> NIPFTDNLLFSGQVLYGDGRLTAKNHQLVMQGDCNLVLYGGKYGWQSNTHGNGEHCFLRLNHKGELIIKDDDFK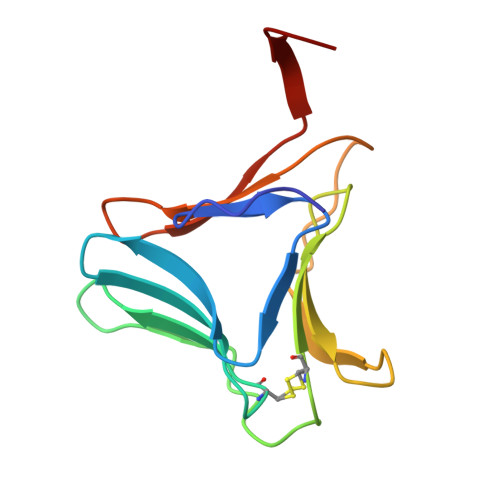TIWSSNSSSKQGDYVLILRDDGFAVIYGPAIWETSA> SNAM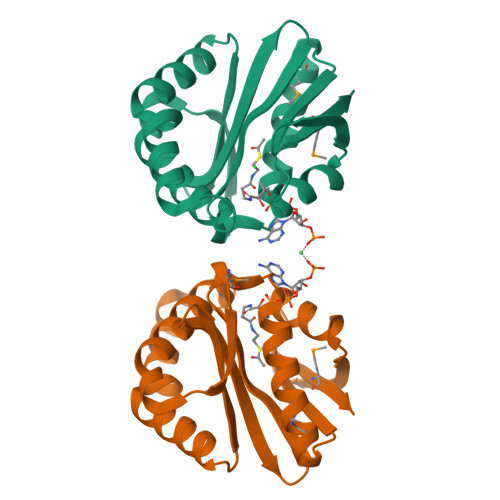SIEIRKLSIEDLETLIEVARESWKWTYAGIYSEEYIESWIREKYSKEKLLNEIVRSQSNLDILFLGAFADSTLIGFIELKIIANKAELLRLYLKPEYTHKKIGKTLLLEAEKIMKKKGILECRLYVHRQNSVGFSFYYKNGFKVEDTDGSDFIMEKKY> DNILYSGETLSTGEFLNYGSFVFIMQEDCNLVL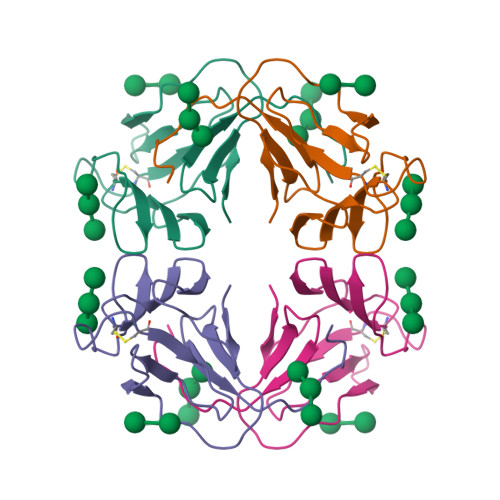YDVDKPIWATNTGGLSRSCFLSMQTDGNLVVYNPSNKPIWASNTGGQNGNYVCILQKDRNVVIYGTDRWATGTHTG ComEA, a DNA-binding protein widely conserved in transformable bacteria, is required for this uptake step. Following this contact with the tpilus, the movement of tDNA into the periplasm is driven by its interaction with the widely conserved periplasmic protein ComEA. A ComEABs contains an N-terminal transmembrane region, a previously unidentified OD, and a C-terminal DNA-binding domain. We show that this domain drives ComEA oligomerization, and that oligomerization is required for genetic transformation.

In contrast to ComEABs, in the ComEAGs structure there was interpretable electron density corresponding not only to the OD (amino acids 62–124) but also to one DNA-binding domain (amino acids 143–207) per asymmetric unit, which contained two OD protomers again arranged head-to-tail. Because there is no interpretable electron density corresponding to the ComEAGs linker region (amino acids 125–142) of either protomer, it is unknown which of the OD monomers in the asymmetric unit OD dimer connects to the single modeled DNA-binding domain. In fact, we could model the DNA-binding domain in the ComEAGs structure only because it made fortuitous crystal contacts. Similarly, in the ComEAGs structure, examination of symmetry mates reveals that the two-membered asymmetric unit uses the OD multimerization interface to form a kinked-ring spiral along the crystallographic screw axis, containing 12 head-to-tail protomers per turn. A slight tilt between ComEAGs protomers has minimal effects on the ComEA inter-dimer bonds, but it causes ComEAGs to form a kinked-ring rather than a closed ring within the crystals. ComEA oligomerization interface amino acids are conserved and mediate conspicuous intermolecular interactions between the OD domains of ComEA protomers, e.g., the side chains of ComEAGs Arg85 and Asp113 (corresponding to ComEABs Arg83 and Asp111) which form intermolecular salt bridges. The ComEAGs X-ray crystal structure revealed not only the structure of the OD, but the three-dimensional shape of the ComEA DNA-binding domain. As predicted from sequence analysis and noted previously, the ComEA DNA-binding domain structure contains two helix-hairpin-helix (HhH) motifs. At an intermediate concentration of 31.3 μM we observed both monomer and dimer, and were able to fit the sedimentation velocity data to a discrete monomer-dimer equilibrium model, resulting in a Kd of 33.8 μM (95% confidence intervals: 19.3 μM, 48.4 μM).

>ASKTAVVDVKGAVANPGVYEVAADARVRDAIALAGGLTDEADETKVNLAAKVHDEMMIYVPKKGEDAPASNAVSKSPSDGDRNGMQVAINTATEEELMQLPGIGPAKANAIIAYREEHGPFRRVEDLLNVTGIGEKTLEKLKPYLLVP[2x]>[2x]SEVDVKDCANHEIKKVLVPGCHGSEPCIIHRGKPFQLEAVFEANQNTKTAKIEIKASIDGLEVDVPGIDPNACHYMKCPLVKGQQYDIKYTWNVPKIAPKSENVVVTVKVMGDDGVLA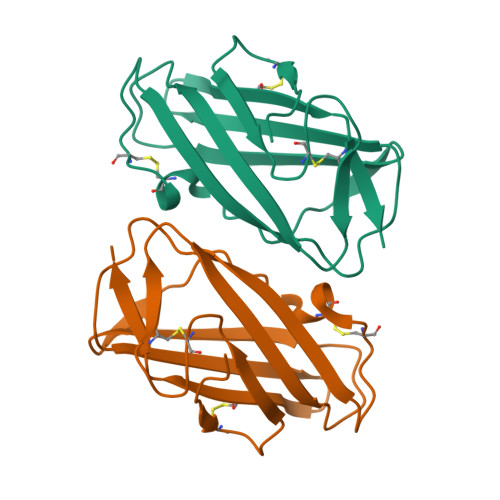CAIATHAKIRD>MRSRRVDVMDVMNRLILAMDLMNRDDALRVTGEVREYIDTVKIGYPLVLSEGMDIIAEFRKRFGCRIIADFKVADIPETNEKICRATFKAGADAIIVHGFPGADSVRACLNVAEEMGREVFLLTEMSHPGA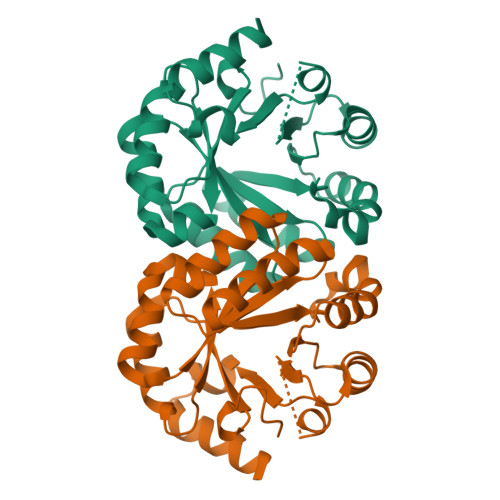EMFIQGAADEIARMGVDLGVKNYVGPSTRPERLSRLREIIGQDSFLISPGVGAQGGDPGETLRFADAIIVGRSIYLADNPAAAAAGIIESIKDLLNP[2x]> MNLAEKMYKAGQI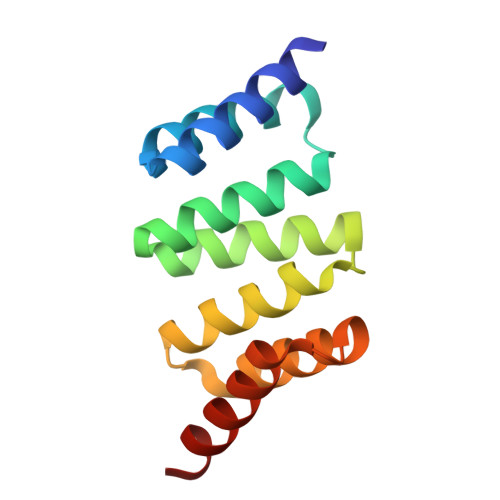EFAKGNYETAIIAYTLALLKDPNNAEAWYNLGEAYLALGNYEEAIEAYQKALELDPNNAEAWYNLGEAYLALGDYDNAIEAFTKALELDPNNKTAKAGLKLAKEKKALE> MLIQIVLVLCQYFQLISCFCQGRLECLNPIQKRCVQIDGLQFIGREKKTGFCVIDSVLYDEIDFCLSESNNVCITYDRKMCIKVESNNSIVAINQEDSICGITIDGYCVDENQNYSQEIYCNDSHCKFTNKQYQKSCLNYKSPQIYGKANKNECVLQDQYFHSDAQIICKPHYCIYFQDKQITCVKMDHSIHPQIIGKDSDGICIFQKVEKQDFYLKYRNLQLCADQKHCYDTSQQTCMPLSASYPAVKMGGTCGNYNEPISISCFYEGNVCLLENPRVCIRIFFNQDYDVCGIRKDGLCAASNIYYQNLQICASDYCMYGQANNAKCIKMDGQQAVGIDSQGFCVQNFEQKADRCSTNFSYICYLNSSQICINLQGYQNYCQQANKCYEFSLQQYIGRDIYYYCIQSEQSLQPQNVQNCLQNPSYICQKRDGTMCVYYYQIPTYFTYLGYINSSGYCAQEGYQTYTSQPQFQTITNLNPNFCQDDSYVIQKILPPYYGRLDSYNYNRCLKQSDQSPYIESCIQGYCISNNSCQKIGFDSKNVSKLSNQYCGLVQQSSAIECAYDQDYCIYNSICYNLSDQNIQTSGIDYYGNCLQRGKYYQNWKKCSVNHCYQKKLLLNSFGCFYLDGTQGAAGIDSNGMCLDYGVSTPVRCALSSQVCLDFQKNTCQQTINFGSTGNGCYYSGYCYQINLGQFIGRDTSLICLSDQEATNNLDTCYNDNQNICMAVYSSLKFCVVYPRTSLYLGYIVQNKQCAVENQQTNQGQLVDLVNLRNNYCQDQQGYIRRLDGKQYVGVDSSQYLCLESGKTPSKSIIQCYTGFCIVENACKAYDQQYVGRDKYYQCLKKGEGISVECAANYCIDLSTKNCVQINDTNPAQAGVLDNFQCAHSERYYYSQILQCSESYCLQQNPNNPSQQGCFELDGDINRAGIDSKGNCLQQDLPNAVRCSPGQFCLNDKFGNACQSLLLSFKNNRFARQKGTGVCLSYIDPSQFKGDNIDICVKGSCKYSDPKNLDFCFSLGQLAFGNQVVGRDINGDCVLKDQQTSTQIVECFDMIYCILDLGGGKQKCQLLQEKDLQFPNLIYKAKNINQTCQDINMPNSMGCLYGLYCINPNDGYKCVLMNDDNKIGRSLVNQQCLQQGELIANYCQPDFCILNGACVPLSNKFPGKENQTQKCLPEQIEGQYGASNCYKEGFCLIINPQNQLASCYQLDYSNPNTIGIQIDTQHCLKEGETVAIMCAYEKYCIDPVSQSCKIQDIKQGYCLGKNGMCAKNGSCVYCQVSQCLTNQNSGTCIDLQQPPALFCKDINVHSENIFIQNQKGICQYLNSGQCDICPENYCKFNNMCFGSQDLLKILKGNQCFVYVPKLKTCQIQDLNTPNSQGNMNCMNNKGFCQDTTVVKNQCLMCANYYFNPGNQQCFSIEEKALLSSSQLFFNMQLIYVKQDCYDQDYCQSIPSLKCPKGCFSCNSPNFCTQCIEGFFLYQDTSNQQFCIQCQKQIIQDNTLKIYYNQIPTYSCLDCSSEYGTWNQISSKYRNCQNFIVKLDNLLQITSQKYAAQNYIISPISTTQAPYQLYFHRSRLCPTGCLSCVQISDSKVMCLQCQDYYINDDNGSCQKCPDFCINCQYATFISGKVIPKSQIEKNQQKYYYFVTICLKCSQYYLVSYNLQSCDNCGINCLYCQYENYKTVLNYN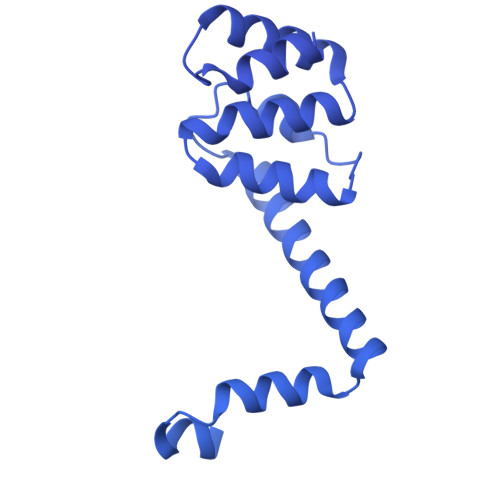IRQLQYLSYYEFSTQNFIKKCIQCPQGYVVGYDGQFCQKEIQNCRYTTFQIAQSYDLTLYIWSFTQNSTIANQICKQCVDGYILSGDASSCLDGCQQQISDNRCESCYSPLNKIQCQFCNSGQILNQVVNPGACQDDICSRNIVGCQECYKYQDPQNPSPFYQIYQCTKCIDQYSIPSIFSCIQCPTGCAKCYEGYRYYNFTSELVYKRTQFTVNQRLNYYQNDYQLYCTECQKGYQFDQQQKKCIKIQCGPNCNLCILINNQPQCVQCNYDKLIAELNQLSYFIGILYFKQNYIPNPKTMISLTSSGNDCQICPILCETCVNNSDVSINPLFIYDAQCLSCKQSLDQSYVLQNYQITYDKSRRKCYLCNKSEQGCYYKKQKVIYAQCLDLSTRLGDGSLQNPINFSRLNEIDLNQFLINEIEYNQAIIYYNELQVKELEVQLIFVDGSCYDYRPQKFSINIKDSIRALSTSLNITTLNQNSVLKFYQLDAFTVQGFDQIYIKNIIFLQQRNDAKLGLILVDKALTNIQLFNCQFLQIQQLIQSIQFMTFNLQTIQQTKVKLEQVVFQNIQIFESTSLININNTQNSSIYLKMNQVKLNNVLFQQSKLISTNSMNITIDITNLFVNQSLFDQQSLLLDMKQNLLVDQYIGILLNNIIFLNSSFLHGSTILNSDFLDFLQIDNLTFNNCTFQQTQKQAVLPLIAANTFMLTQIQIISNTITNYSFLQQYDNYFKDQNQSSSFSGIDIIDNKVNSDSYLFLFFQTQQNRNSSIHGINILRNQFSSNYTQVIVQFNQQNFVQIQNLTIVDNQQFLFISTDSVRNILLQQVYQYQTSSQYFAAQICYLRQTKNQINIKNIKLEGIYFQKNIFQIENSLNNYLQKDFQITVTNLFSTQSTLLLKRYTNDVTIFSLYSKQQISLTVQNVTFSFFKSQVLNNKTSLGKISLGFYFQGLQIKATILNSTFADLDISSPFNWIEGSVQQMILKSCNFTNSNGYQNYNSVRNGGFFKITSQKLIIKKSIFINGNALNGGAFYLIMQGKGTLNLINSTFINNKAYSNNDQETKGGAFYLDGFMSESLDVLVFKSIFSKNLALFSGGAINIQSSNQQNAFIIQESFFFDNLSCQGSSINIQSSSDFQSEVVISKTKVNNQIQNTISTVENIANLLSQYTLLNIQQLSSSQIFIKDVRNVQFFQSRFQIVPYKFKDSNVLKYFKGIIFSQMFSIQNVLNYLDINNIYEKSVFYGKLINVNNVKNIQIQHTQILNNQNIIEDLSHQDNRVSNLASFHSQNCLVFNLTVNQNKCLQCNLGIIEILSSKLDMQNSTFQNNLAQYGSSLQLQQNKQYIYNLSKLLQSFQDKLVISNSTFSHNIANVNGGALYIKESTVFIYQTLFDTNTARQYGGALFLENTKKNILTNLINLQNCTFSNNKAKFGGVLASTTGQRVNKYTNNTYKDNKGYQYGENIQTSPTKFIITVNKTQLTDTQYINIQNHQGGTLRDEILLALCDDQNNYIQNIPQDSFLSINITQGSGFLNQNKIAHKNGIFNLTQQIQVYGYSKQQLLLSITSDLIQIPVFNKDEIIIGYDSYQLIINIQMVQVCLPGQIPKKFQEKFDLCYDCQDGSYSFQVSDTCQICPSPQAKCFRDKILLPSNLWRVSQKSIVLFPCKNCVGDIQLYKKFKKRSLLKIQSTDLNYYCKEGYIGALCEDCDRNGQHWGDSYFMNLDLKCQRCSQTTFAEIAYPLMISLIAFILMIFLTYYIQIQVHLKLTKKVLTILSKKYYGFNDQSIARTIKFLVYQSSIIGIMFWYDCYIPNTFSYIFIDIGNLFTDQIRISECFLEQKFSGTSIIYKGIYFLLGTYFAIISCIIIFYMLLRIKFNYQNYLQDILISLSIFVYFSYNSILSKIFRSVIHLLFLKIKKNVILQNITNRLIAKSLTKKDSQWSIYQFHVMK>[2x]GLEHCVKIIRQLECSGHIDKNFRQKFLTWYS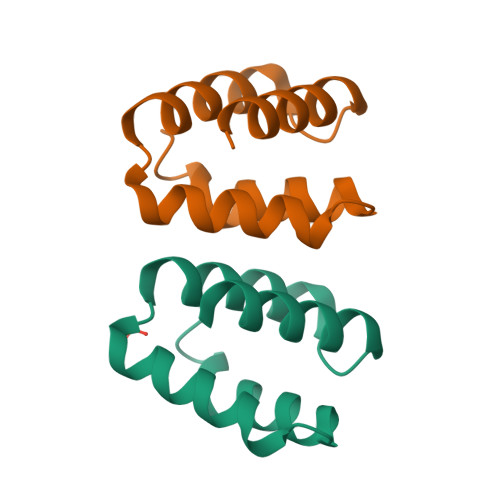LRATSQEIRVVKDFIDTFIDDPMALAEQLIDTFDDRVS>MDKNPQPQAQQTTQTTTTAAGSAADQGVPASGQGKLISVKTDVLDLTINTRGGDVEQALLPAYPKELNSTQPFQLLETSPQFIYQAQSGLTGRDGPDNPANGPRPLYNVEKDAYVLAEGQNELQVPMTYTDAAGNTFTKTFVLKRGDYAVNVNYNVQNAGEKPLEISSFGQLKQSITLPPHLDTGSSNFALHTFRGAAYSTPDAAYAAYAFDTIADNENLNIS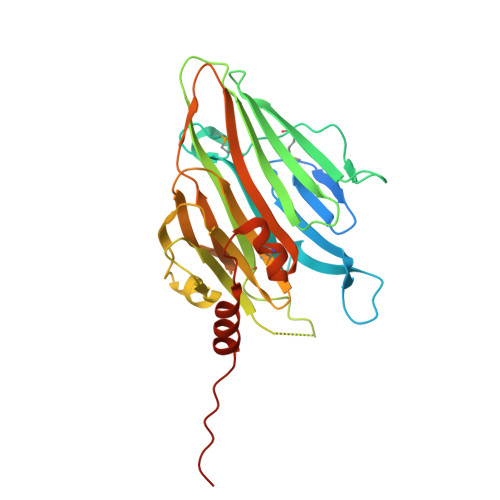SKGGWVAMLQQYFATAWIPHNDGTNNFYTANLGNGIAAIGYKSQPVLVQPGQTGAMNSTLWVGPEIQDKMAAVAPHLDLTVDYGWLWFISQPLLVPRGSLEHHHHHH[2x]5-[[(2S)-2-[[(3R,4S)-5-(3,5-difluorophenoxy)-3-hydroxy-4-[[3-(methyl-methylsulfonyl-amino)-5-[[(1R)-1-phenylethyl]carbamoyl]phenyl]carbonylamino]pentanoyl]amino]-3-methyl-butanoyl]amino]benzene-1,3-dicarboxylic acid | C42 H45 F2 N5 O12 S | 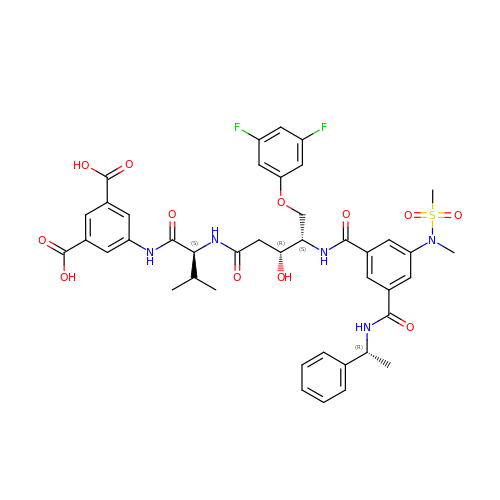XYKCBRCSBVZGIL-WRXYKUNKSA-N>[3x]MTTADLILINNWHVVANVEDCKPGSITTARLLGVKLVLWRSQEQNSPIQVWQDYCPHRGVPLSMGEVANNTLVCPYHGWRYNQAGKCVQIPAHPDMVPPASAQAKTYHCQERYGLVWVCLGNPVNDIPSFPEWDDPNYHKTYTKSYLIQASPFRVMDNSIDVSHFPFIHDGWLGDRNYTKVEDFEVKVDKDGLTMGKYQFQTSRIVSHIEDDSWVNW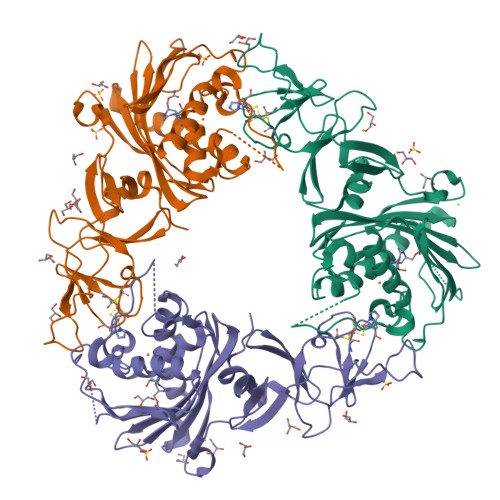FRLSHPLCQYCVSESPEMRIVDLMTIAPIDEDNSVLRMLIMWNGSEMLESKMLTEYDETIEQDIRILHSQQPARLPLLAPKQINTQGLPQEIHVPSDRGTVAYRRWLKELGVTYGVC> GPDEARRQIVSNALISEIAGIVDFVAEEQITVIEQGIEKEITNPLYEQSSGIPYINRTTNKDLNSTMSTNASEFINWGAGTSTRIFFTRKYCISTGTQGNYEFSKDYIPCEEPAILSNSDLKIDRIDFVATDNTVGSAIERVDFILTFDKSNANESFYFSNYVSSLEKAAEQHSISFKDIYVVERNSSGAAGWRLTTISGKPLTFSGLSKNIGSLDKTKNYGLRLSIDPNLGKFLRADGRVGADKLCWNIDNKMSGPCLAADDSGNNLVLTKGKGAKSNEPGLCWDLNTGTSKLCLTQIEGKDNNDKDASLIKLKDDNGNPATMLANILVEEKSMTDSTKKELRTIPNTIYAAFSNSNASDLVITNPGNYIGNVTSEKGRIELNVQD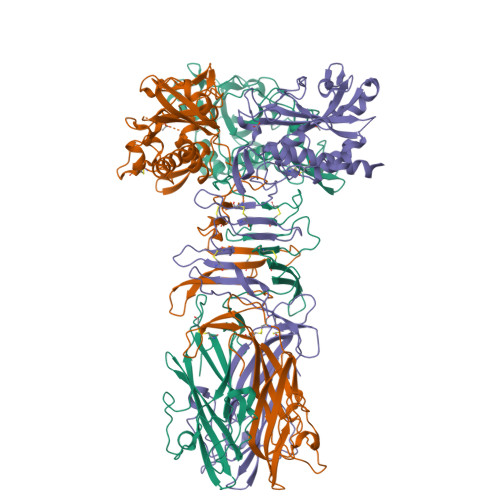CPVSPDGNKLHPRLSASIASIVADTKDSNGKYQADFSSLAGNRNSGGQLGYLSGTAIQVNQSGSKWYITATMGVFDPLTNTTYVYLNPKFLSVNITTWCSTEPQT>[2x]GADPKKVLDQAKDQMENVVRTLKQELEELAKEARKLDLTQSEKIELKLRYIVAHLAAIGDIEEAIREAKEEADKLKRAGLVNSQQFDEFKRRLEELHKEADRKRADYAEEFRNKLEYG

BCL-2 protein family members BAK and BAX are the gatekeepers of mitochondrial apoptosis. Homooligomers of BAK and BAX form pores in the mitochondrial outer membrane (MOM) and release apoptotic factors into the cytosol, committing the cell to destruction. We use computational protein design to generate high affinity binders of BAK and BAX with greater than 100-fold specificity for their target. Both binders activate their targets when at low concentration, driving pore formation, but inhibit membrane permeabilization when in excess.

As a starting point for design, we used as a scaffold a de novo designed protein BINDI that binds with high affinity to BHRF1, a viral prosurvival BCL-2 homolog. BINDI has high stability (resistance to thermal and chemical denaturation) and therefore is likely to be tolerant of the mutations necessary to enable interaction with BAK and BAX, and we demonstrated previously that the three-helix structure of BINDI can be redesigned for altered BCL-2 family specificity. During the design and evolution of αBAK2, we generated two lower affinity constructs for BAK, αBAK1, and CDP02, which bound to BAK with Kd values of 7 and 60 nM respectively. Five rounds of FACS under specificity-enriching conditions yielded binders with high affinity and specificity. αBAK2 binds BAK with 400 ± 200 pM affinity and 333-fold specificity. αBAX2 binds BAX with 3 ± 2 nM affinity and 100-fold specificity. αBAK2 differs by 12 mutations (10%) from precursor αBAK1 and 22 mutations (19%) from BAK-CDP02. αBAX2 differs by 10 mutations (9%) from precursor αBAX1 and 18 mutations (15%) from BAX-CDP01. Crystal structures agree with the computational model and confirm the BH3-mimetic binding mode of αBAK2 with BAK.N-hydroxy-N~2~-{[2-(4-methoxyphenyl)ethyl]sulfonyl}glycinamide 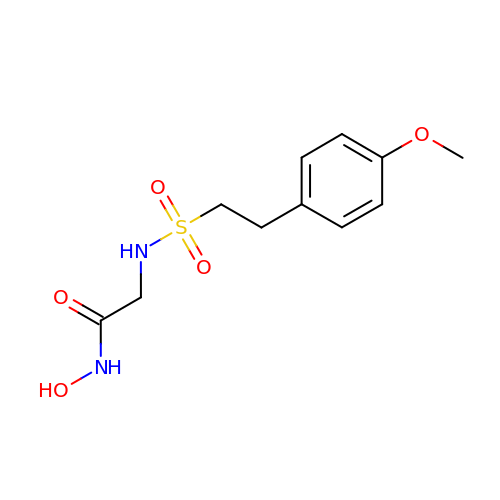| C11 H16 N2 O5 S | LMKSZZKXCRCXFM-UHFFFAOYSA-N> MNSITVRNATFTWARSDPPTLNGITFSIPEGALVAVVGQVGCGKSSLLSALLAEMDKVEGHVAIKGSVAYVPQQAWIQNDSLRENILFGCQLEEPYYRSVIQACALLPDLEILPSGDRTEIGEKGVNLSGGQKQRVSLARAVYSNADIYLFDDPLSAVDAHVGKHIFENVIGPKGMLKNKTRILVTHSMSYLPQVDVIIVMSGGKISEMGSY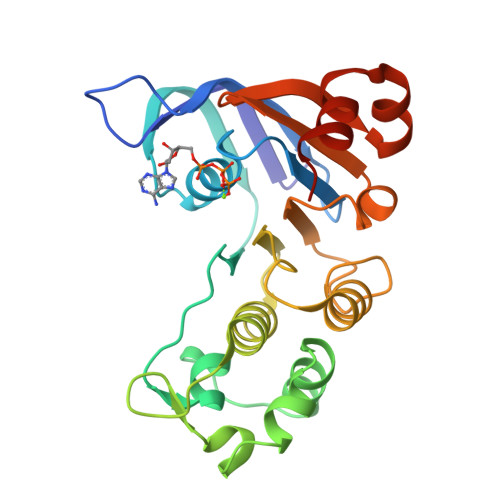QELLARDGAFAEFLRTYASHHHHHH>XAATSRPERVWPDGVIPFVIGGNFTGSQRAVFRQAMRHWEKHTCVTFLERTDEDSYIVFTYRPCGCCSYVGRRGGGPQAISIGKNCDKFGIVVHELGHVVGFWHEHTRPDRDRHVSIVRENIQPGQEYNFLKMEPQEVESLGETYDFDSIMHYARN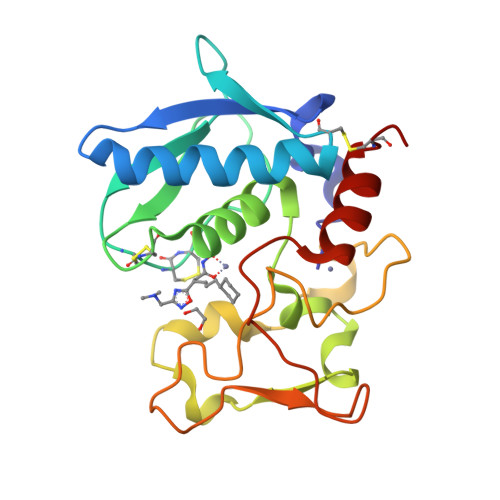TFSRGIFLDTIVPKYEVNGVKPPIGQRTRLSKGDIAQARKLYKCPA[2x]A genetically unrelated functional amyloid protein system (Fap) is found in many β-, δ-, and γ-proteobacteria and in pathogenic strains and is thought to function as a virulence enhancing factor. The major fiber-forming subunits are FapB and FapC, which are exported across the outer membrane via the membrane protein FapF, along with FapE which is also detected as a minor component associated with Fap fibers. Full-length FapF possesses a large N-terminal periplasmic region comprising the first 70-amino-acid residues. In vivo secretion assays have demonstrated that this periplasmic domain is essential for secretion by regulating the release of the helical plug.

Using a combination of X-ray crystallography and solution NMR spectroscopy together with molecular dynamics simulations, we show that the coiled coil forms a novel asymmetric trimer of parallel helices. Crystals were only observed to form in two zinc acetate containing conditions over 3–5 days of which only one was of suitable diffraction quality [JSCG + 0.2 M zinc acetate dihydrate, 0.1 M sodium cacodylate (pH 6.5), 10% v/v 2-propanol]. We therefore subsequently processed the diffraction data in P1 to model the six chains in the asymmetric unit individually and the structure could be refined using REFMAC5 and PHENIX with a final Rfree of 24%. One trimer (chains ABC) was fully resolved, whereas for the second (chains DEF), the termini could not be fully resolved. As the 1H–1H NOESY spectra clearly show three tyrosine residues in distinct conformations that are not exchanging on the NMR timescale, we were able to confidently model the core of the coiled coil with a single buried Tyr20 side chain per trimer. The final geometry of the three tyrosines within the crystal structure is also consistent with the NOE correlations between upfield shifted methyl groups of the Leu16 and Tyr20 side-chains protons. This leads to an asymmetric arrangement of two surface-exposed tyrosine residues within the trimer and the configuration allows the buried Tyr20 side chain to coordinate with a Gln23 side chain of an adjacent chain. Despite the asymmetry of the central tyrosine residues, the conformation of the backbone for the three peptide chains is symmetric, as the number of backbone amides peaks observed in the 1H–15N heteronuclear single quantum coherence spectroscopy (HSQC) NMR spectrum is consistent that expected for single peptide chain. Another striking feature of FapFCC is the presence of the buried polar Gln23 residues, which are stabilized by neighboring Gln24 residues through an extended hydrogen bonded network across the core of the protein. Furthermore, asymmetry in the surface properties of FapFCC could enable the recruitment of other Fap proteins in a sub-stoichiometric ratio. It is worth noting that much of the surface is polar as expected; however, the central portion of the protein displays a surface hydrophobic pocket that could represent a key binding site.

>DVDIETLKQELLELKQRYEAQQKALAVLEQRVRQVEDQ[6x]> K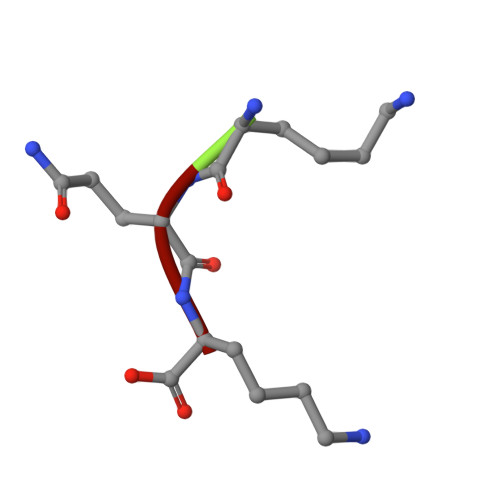QK> MAYLEQLQAGLRYLGRAGESGRKSLDKVVAPVNGAISEIRGAAAELENLPGVSPEMAARLQRAMRGIGQAQGKVNRVVSTYDRASRALLGIDERLDALKVQVNSAAQAVG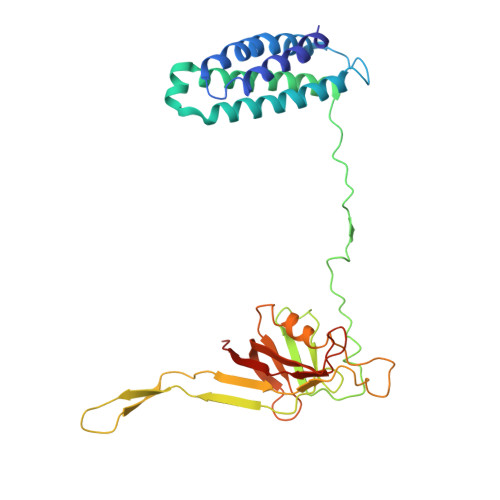KVAGDISPTLAGVLPSWLLAPSATPPSEAAASLPHLLVLQPLTANAQPFYFNLNTAAFDALQRNSAYNWSGQVRLGRRPALQSVGMGEESILLKGAVFPLRRQVGNQEKVVGLEQLEALRRLAERREPLILSSGYGEVQMGLWCLVRISENQSALLGNGAPRKQTFDLEFKRYGDDLPNR KCR channelrhodopsins (K+-selective light-gated ion channels) have received attention as potential inhibitory optogenetic tools but more broadly pose a fundamental mystery regarding how their K+ selectivity is achieved. Here, we present 2.5–2.7 Å cryo-electron microscopy structures of HcKCR1 and HcKCR2 and of a structure-guided mutant with enhanced K+ selectivity. Structural, electrophysiological, computational, spectroscopic, and biochemical analyses reveal a distinctive mechanism for K+ selectivity; rather than forming the symmetrical filter of canonical K+ channels achieving both selectivity and dehydration, instead, three extracellular-vestibule residues within each monomer form a flexible asymmetric selectivity gate, while a distinct dehydration pathway extends intracellularly.

In HcKCR2, the N-terminal P2 is surrounded by P95, F96, W100, and Y101 with no space for the first methionine, consistent with its predicted post-translational cleavage. The overall structures of HcKCR1 and 2 are almost identical with only minor differences in the N-terminal region, ICLs, and ECLs. HcKCR1 and 2 exhibit different spectral properties; λmax of HcKCR1 and 2 are 521 nm and 486 nm, respectively. Despite similarity in retinal binding pockets, these differ at positions 136 and 140 near the β-ionone ring of the retinal, offering an opportunity to investigate spectral mechanisms. While 6-s-trans-retinal is found in all reported structures of naturally occurring microbial rhodopsins, during the structural refinement of HcKCR2 with 6-s-trans-retinal (STAR Methods), we observed a steric clash between the C17 atom of retinal and the methyl group of A140, along with extra density next to the C18 atom (top). Modeling 6-s-cis-retinal resolved this issue (bottom), indicating that these two residues (A136/A140 in HcKCR2) create a steric clash with the C17 atom and simultaneously make space to accommodate the C16 atom to induce the rotation of the β-ion-one ring. The ~220° rotation of the ring shrinks the π-conjugated system of retinal and thereby induces a ~35 nm spectral shift. Swapping these two residues between HcKCR1 and HcKCR2 confirmed their influence on the orientation of the β-ionone ring and largely explained the spectral difference. HcKCR2 thus represents the initial naturally occurring microbial rhodopsin with experimentally demonstrated 6-s-cis-retinal configuration. Two residues (T136/G140 in HcKCR1 and A136/A140 in HcKCR2) are involved in the conversion, and considering a previous study with the C1C2 chimera, G-to-A-replacement at position 140 could be sufficient for the conversion, while position 136 may fine-tune the twist.

> MPFYDSRPPEGWPRGSVNDMDYPLLGSICAISAIAIAGSGIWMLYRLDLGMGYSCKPYKSGRAPEVNSISGIVCLLCGTMYAAKSFDFFDGGGTPFSLNWYWYLDYVFTCPLLIVDFAFTLDIPQKLRYSIAVFVALWCAVAAFATPSAFRFAYYALGCCWFIPLSLFLIRDVKKRYQVYPPKCQRLLFWACVVFFGFWPLFPLLFIFSWQGSGHISRQAYYIIHAFLDLVCKSIFGFLMTFFRLELEEHTEVQGLPLKEPKVMDAAAKSRITSEGEYIPLDQIDINVGAPGSSLEVLFQ>HGYVESPASRAYQCKLQLNTQCGSVQAEPQSVEGLKGFPQAGPADGHIASADKSTFFELDQQT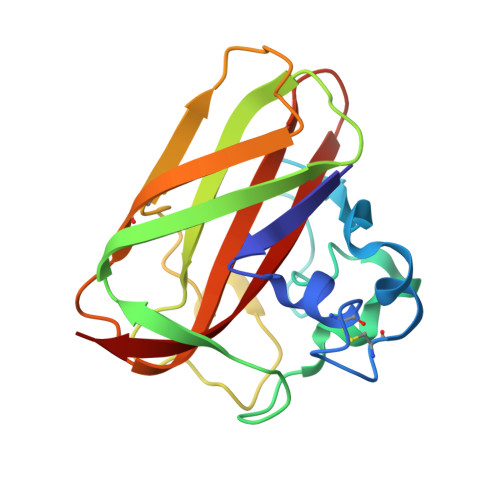PTRWNKLNLKTGPNSFTWKLTARHSTTSWRYFITKPNWDASQPLTRASFDLTPFCQFNDGGAIPAAQVTHQCNIPADRSGSHVILAVWDIADTANAFYQAIDVNLSK[2x]>[60x]MNTKKMLKEYNKKVKRKGLAGLDTAIILIAFIITASVLAYVAINMGLFVTQKAKSTINKGEETASTALTLSGSVLYAVNYPSNTRSYWIYFTVSPSSGVSSVELSPSTTAISFTASAEGISYSNIYEYTLLTVSPSELANQVYANGQYLDLVNQQTNAGQTY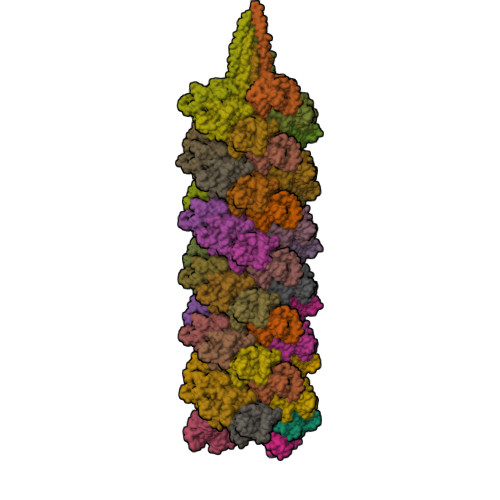VYYPNPYYALLALNYTLSKIDKVSPSPLYITTTTPSSATQIYPFLAHDNMFTFTLNISGTLVTYYAFVNQTFAFTYPVAGDPLIGSAIAPAGSVIGVMILFGPDLGSHVFQYQTITIQITPNIGSPLTISEYVYQPEGSVSVIG7-METHYLGUANOSINE | C11 H16 N5 O5 | 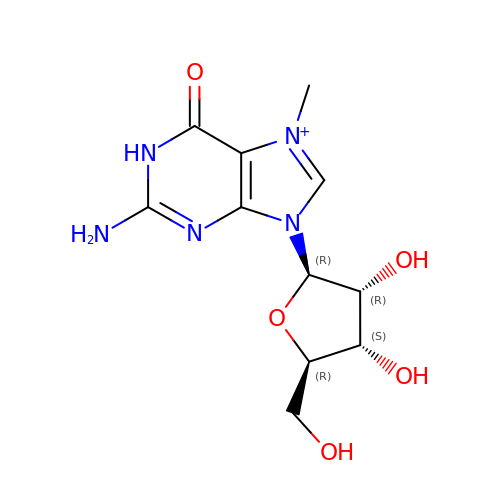OGHAROSJZRTIOK-KQYNXXCUSA-O> PISPIETVPVKLKPGMDGPKVKQWPLTEEKIKALVEICTEMEKEGKISKIGPENPYNTPVFAIKKKDSTKWRKLVDFRELNKRTQDFWEVQLGIPHPAGLKKKKSVTVLDVGDAYFSVPLDEDFRKYTAFTIPSINNETPGIRYQYNVLPQGWKGSPAIFQSSMTKILEPFRKQNPDIVIYQYMDDLYVGSDLEIGQHRTKIEELRQHLLRWGLTTPDKKHQKEPPFLWMGYELHPDKWTVQPIVLPEKDSWTVNDIQKLVGKLNWASQIYPGIKVRQLSKLLRGTKALTEVIPLTEEAELELAENREILKEPVHGVYYDPSKDLI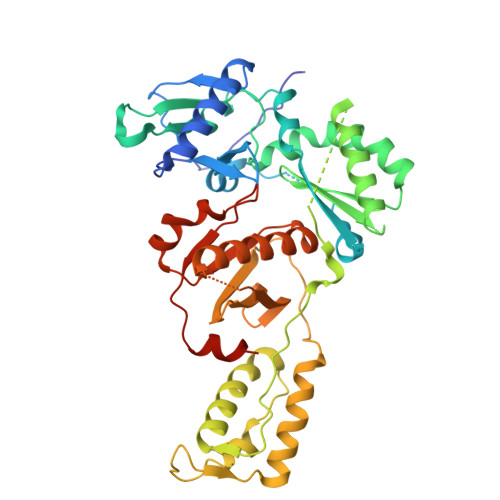AEIQKQGQGQWTYQIYQEPFKNLKTGKYARMRGAHTNDVKQLTEAVQKITTESIVIWGKTPKFKLPIQKETWETWWTEYWQATWIPEWEFVNTPPLVKLWYQLEKEPIVGAETF> MILFDKNKRILKKYAKMVSKINQIESDLRSKKNSELIRLSMVLKEKVNSFEDADEHLFEAFALVREAARRTLGMRPFDVQVMGGIALHEGKVAEMKTGEGKTLAATMPIYLNALIGKGVHLVTVNDYLARRDALWMGPVYLFLGLRVGVINSLGKSYEVVWKNPDLARKAIEENWSVWPDGFNGEVLKEESMNKEAVEAFQVELKEITRKEAYLCDVTYGTNNEFGFDYLRDNLVLDYNDKVQRGHFYAIVDEADSVLIDEARTPLIISGPSKESPSVYRRFAQIAKKFVKDKDFTVDEKARTIILTEEGVAKAEKIIGVENLYDPGNVSLLYHLINALKALHLFKKDVDYVVMNGEVIIVDEFTGRLLPGRRYSGGLHQAIEAKEGVPIK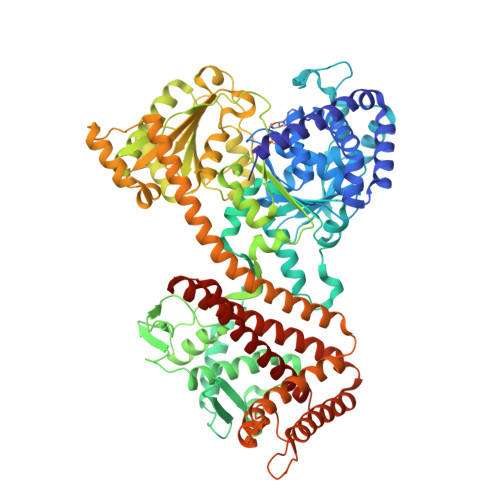EESITYATITFQNYFRMYEKLAGMTGTAKTEESEFVQVYGMEVVVIPTHKPMIRKDHDDLVFRTQKEKYEKIVEEIEKRYKKGQPVLVGTTSIEKSELLSSMLKKKGIPHQVLNAKYHEKEAEIVAKAGQKGMVTIATNMAGRGTDIKLGPGVAELGGLCIIGTERHESRRIDNQLRGRAGRQGDPGESIFFLSLEDDLLRIFGSEQIGKVMNILKIEEGQPIQHPMLSKLIENIQKKVEGINFSIRKTLMEMDDVLDKQRRAVYSLRDQILLEKDYDEYLKDIFEDVVSTRVEEFCSGKNWDIESLKNSLSFFPAGLFDLDEKQFSSSEELHDYLFNRLWEEYQRKKQEIGEDYRKVIRFLMLRIIDDHWRRYLEEVEHVKEAVQLRSYGQKDPIVEFKKETYYMFDEMMRRINDTIANYVLRVLEHHHHHH>[2x]GHMASGPWKLTASKTHIMKSADVEKLADELHMPSLPEMMFGDNVLRIQHGSGFGIEFNATDALRCVNNYQGMLKVACAEEWQESRTEGEHSKEVIKPYDWTYTTDYKGTLLGESLKLKVVPTTDHIDTEKLKAREQIKFFEEVLLFEDELHDHGVSSLSVKIRVMPSSFFLLLRFFLRIDGVLIRMNDTRLYHEADKTYMLREYTSRESKISSLMHVPPSLFTEPNEISQYLPIKEAVCEKLIFPE;>ENLYFQ[2x]

TIPRL (TIP41, TOR signaling pathway regulator-like) is a type 2A phosphatase regulatory protein which is still poorly understood both structurally and functionally. In a previous study, we performed a yeast two-hybrid screen using human TIPRL as bait and found that it binds the catalytic subunits of PP2A, PP4 and PP6 and inhibits the activity of PP2A in vitro. However, contrary to the yeast Tip41, which inhibits TOR signaling by sequestering the α4 orthologue Tap42, human TIPRL positively regulates mTORC1 signaling in response to amino acids. The TIPRL interaction surface on PP2Ac includes the active site and overlaps with the binding surfaces for LCMT1, PTPA and PME-1, supporting a role for TIPRL in PP2A biogenesis or recycling.

Here, we report the crystal structure of human TIPRL, revealing a novel protein fold bound to a TEV site-derived peptide which mimics the conserved C-terminus of PP2Ac. The structure obtained through selenomethionine experimental phasing consists of a new fold of α-helices and 310 helices organized around a beta-sandwich core in a unique topology. The last 16 C-terminal residues of TIPRL show no electron density in the crystal structure, indicating structural disorder. The asymmetric unit of the crystal contained two molecules that seem to form a dimer. The β-strand in the N-terminus of TIPRLΔN (β1) is critical to form the dimer interface in the asymmetric unit and its amino acid residues originate from a plasmid-derived sequence instead of TIPRL itself (GHMAS), agreeing with the fact that the full length TIPRL construct does not dimerize. The density maps of both molecules in the asymmetric unit present a positive electron density inside the bottom cleft that cannot be accounted by the TIPRL sequence. This positive density can be correctly modeled as the four C-terminal residues from the TEV cleavage site, LYFQ, bound to the TIPRL chain A. The same peptide was bound to the symmetric binding site on chain B and stabilized by further interactions with chain A, which allowed for the modelling of the entire TEV site, ENLYFQ. The binding site for the peptide shows alternating patches of hydrophobic (I147/F150 and L141/L182) and positively charged residues (K171/R173 and R184/R200). One major exception is R200, which engages in ionic interactions with the C-terminal carboxylate group.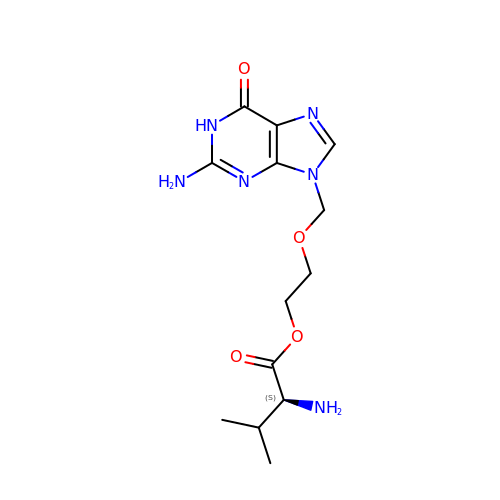2-[(2-amino-6-oxo-1,6-dihydro-9H-purin-9-yl)methoxy]ethyl L-valinate | C13 H20 N6 O4 | HDOVUKNUBWVHOX-QMMMGPOBSA-N>[6x]MRGSHHHHHHGSMDKNIIIGAMTALITPFKNGKVDEQSYARLIKRQIENGIDAVVPVGTTGESATLTHEEKRTCIEIAVETCKGTKVKVLAGAGSNATHEAVGLAKFAKEHGADGILSVAPYYNKPTQQGLYEHYKAIAQSVDIPVLLYNVPGRTGCEISTDTIIKLFRDCENIYGVKEASGNIDKCVDLLAHEPRMMLISGEDAINYPILSNGGKGVISVTSNLLPDMISALTHFALDENYK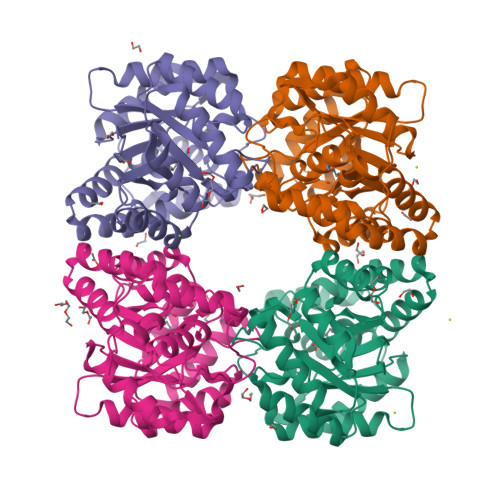EAKKINDELYNINKILFCESNPIPIKTAMYLAGLIESLEFRLPLCSPSKENFAKIEEVMKKYKIKGF> MEQRETIMLPGSDYNHWLIVMEFPKDPAPSRDQMIDTYLNTLATVLGSMEEAKKNMYAFSTTTYTGFQCTIDEETSEKFKGLPGVLWVLPD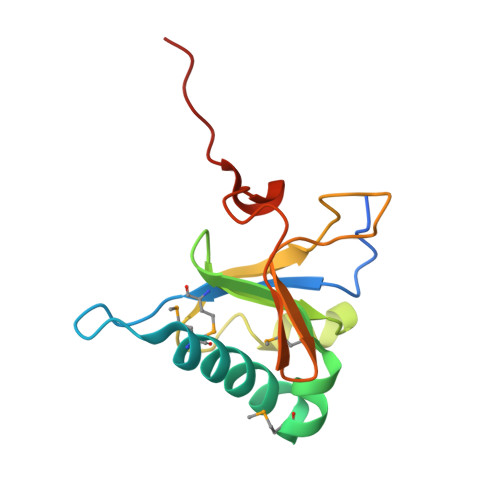SYIDVKNKDYGGDKYINGEIIPSTYPTYQPKQLEHHHHHHHH> MSEMQGNKIVVDPITRIEGHLRIEVEVEGGKIKNAWSMSTLFRGLEMILKGRDPRDAQHFTQRACGVCTYVHALASVRAVDNCVGVKIPENATLMRNLTMGAQYMHDHLVHFYHLHALDWVNVANALNADPAKAARLANDLSPKKTTTESLKAVQAKVKALVESGQLGIFTNAYFLGGHPAYVLPAEVDL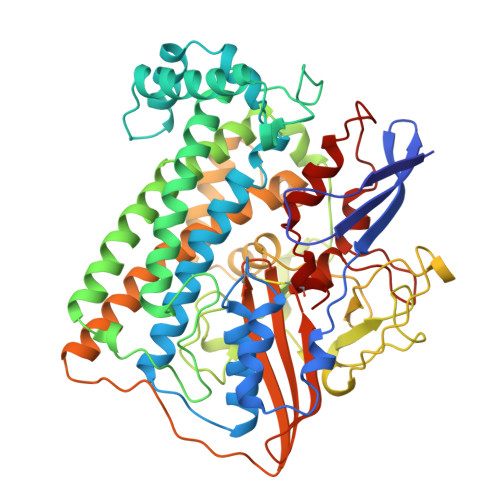IATAHYLEALRVQVKAARAMAIFGAKNPHTQFTVVGGCTNYDSLRPERIAEFRKLYKEVREFIEQVYITDLLAVAGFYKNWAGIGKTSNFLTCGEFPTDEYDLNSRYTPQGVIWGNDLSKVDDFNPDLIEEHVKYSWYEGAGAHHPYKGVTKPKWTEFHGEDRYSWMKAPRYKGEAFEVGPLASVLVAYAKKHEPTVKAVDLVLKTLGVGPEALFSTLGRTAARGIQCLTAAQEVEVWLDKLEANVKAGKDDLYTDWQYPTESQGVGFVNAPRGMLSHWIVQRGGKIENFQLVVPSTWNLGPRCAEGKLSAVEQALIGTPIADPKRPVEILRTVHSYDPCIACGVH> GSRSEPAKVVDIRIDTSAERKPISPYIYGSNQELDATVTAKRFGGNRTTGYNWENNFSNAGSDWLHYSDTYLLEDGGVPKGEWSTPASVVTTFHDKALSKNVPYTLITLQAAGYVSADGNGPVSQEETAPSSRWKEVKFEKGAPFSLTPDTEDDYVYMDEFVNYLVNKYGNASTPTGIKGYSIDNQPALWSHTHPRIHPDNVTAKELIEKSVALSKAVKKVDPYAEIFGPALYGFAAYETLQSAPDWGTEGEGYRWFIDYYLDKMKKASDEEGKRLLDVL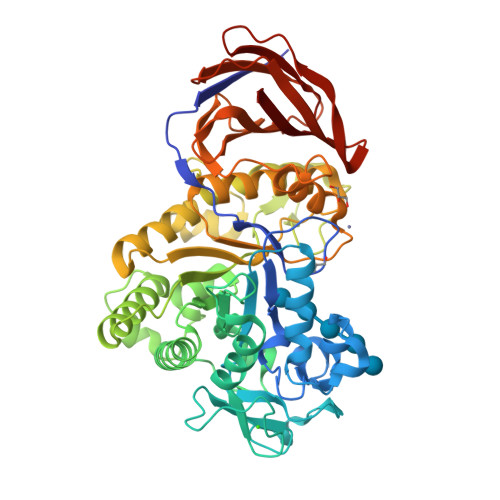DVHWYPEARGGGERICFGADPRNIETNKARLQAPRTLWDPTYIEDSWIGQWKKDFLPILPNLLDSIEKYYPGTKLAITEYDYGGGNHITGGIAQADVLGIFGKYGVYLATFWGDASNNYTEAGINLYTNYDGKGGKFGDTSVKCETSDIEVSSAYASIVGEDDSKLHIILLNKNYDQPTTFNFSIDSSKNYTIGNVWAFDRGSSNITQRTPIVNIKDNTFTYTVPALTACHIVLEAAEP> KHTLPDLPFDYADLEPVISHEIMQLHHQKQHATYVNNLNQIEEKLHEAVSKGNLKEAIALQPALKFNGGGHINHSIFWTNLAK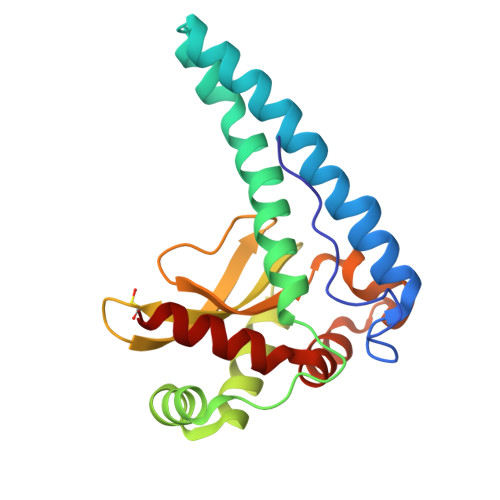DGGEPSKELMDTIKRDFGSLDNLQKRLSDITIAVQGSGWGWLGYCKKDKILKIATCANQDPLEGMVPLFGIDVWEHAYYLQYKNVRPDYVHAIWKIANWKNISERFANARQ> GPVEESVDRAVARVADTISSRPTNSESIPALTAAETGHTSQVVPSDTMQTRHVKNYHSRSESSIENFLCRSACVYYATYTNNSKKGFAEWVINTRQVAQLRRKLELFTYLRFDLELTFVITSAQQPSTASSVDAPVQTHQIMYVPPGGPVPTKVKDYAWQTSTNPSVFWTEGNAPPRMSIPFISIGNAYSCFYDGWT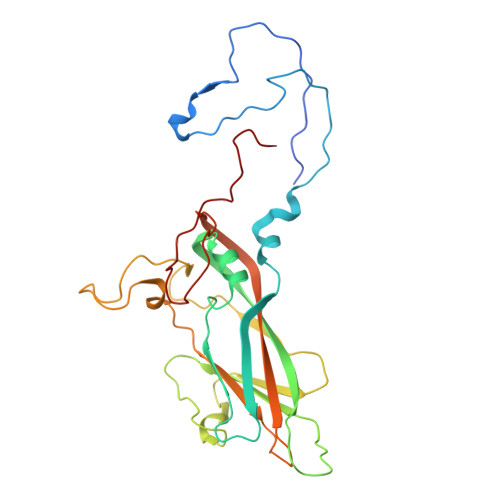QFSRNGVYGINTLNNMGTLYMRHVNEAGQGPIKSTVRIYFKPKHVKAWVPRPPRLCQYEKQKNVNFSPIGVTTSRTDIITT> MAFSELLDQVGGLGRFQVLQTVALVVPIMWLCTQSMLENFSAAVPSHRCWVPLLDNSTAQASVPGALGPEALLAVSIPPGPNQGPHQCRRFRQPQWQLLDPNATATNWSEAATEPCVDGWVYDRSTFTSTIVAKWDLVCDSQALKPMAQSIYLAGILVGAAVCGPASDRFGRRLVLTWSYLQMAVSGTAAAFAPTFPVYCLFRFLVAFAVAGVMMNTGTLVMEWTSAQARPLVMTLNSLGFSFGHVLMAAVAYGVRDWALLQLVVSVPFFLCFVYSCWLAESARWLLITGRLDRGLRELQRVAAINGKRAVGDTLTPQVLLSAMQEELSVGQAPASLGTLLRTPGLRLRTCISTLCWFAFGFTFFGLALDLQALGSNIFLLQVLIGVVDIPAKIGTLLLLSRLGRRPTQAASLVLAGLCILANTLVPHEMGALRSALAVLGLGGLGAAFTCITIYSGELFPTVLRMTAVGLGQMAAR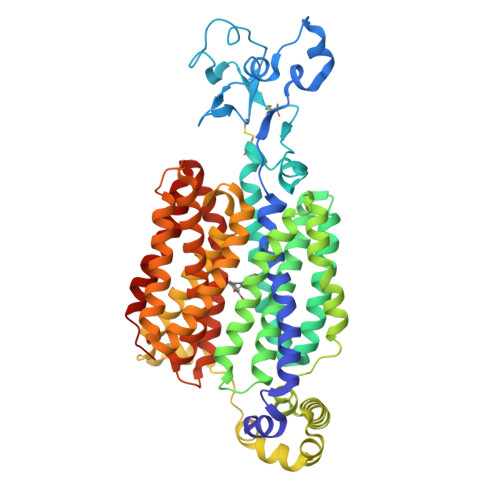GGAILGPLVRLLGVHGPWLPLLVYGTVPVLSGLAALLLPET>[3x]GACDNDTEPGGTAVEKMAGDWWVTVNAFIDGKEVEDPFGAGHLQMSTYNTASNSETEMWLDDLGNFWEYKLKVNVNYAARTFSTTGFVDNVTYESKVK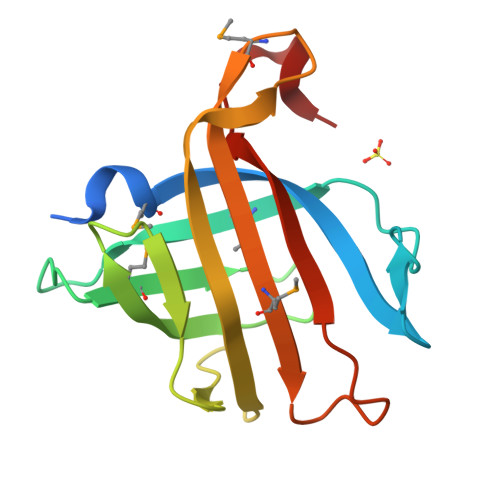ITDGKVLEKAATTPSGMPADSIVYMVQFDDDEDGLTYKVSGFRRTGFPADDF> GAMGSIKEIAITHHVKEGHEKADPSQFELLKVLGQGSFGKVFLVKKISGSDARQLYAMKVLKKATLKVRDRVRTKMERDILVEVNHPFIVKLHYAFQTEGKLYLIL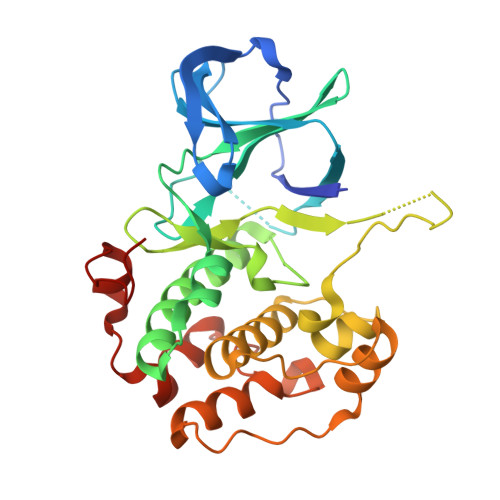DFLRGGDLFTRLSKEVMFTEEDVKFYLAELALALDHLHSLGIIYRDLKPENILLDEEGHIKLTDFGLSKESIDHEKKAYSFCGTVEYMAPEVVNRRGHTQSADWWSFGVLMFEMLTGTLPFQGKDRKETMTMILKAKLGMPQFLSPEAQSLLRMLFKRNPANRLGAGPDGVEEIKRHSFFSTIDWNKLYRREIHPPFKP>[2x]TYKITVRVYQTNPDAFFHPVEKTVWKYANGGTWTITDDQHVLTMGGSGTSGTLRFHADNGESFTATFGVHNYKRWCDIVTNLAADETGMVINQQYYSQKNREEARERQLSNYQVKNAKGRNF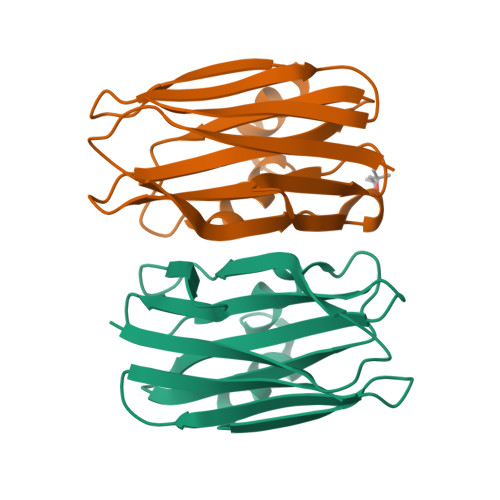QIVYTEAEGNDLHANLIIG> GPLGSPNSEEEASVSVWDEEEDGATFTVTSRQYRPLDPLAPLPPPRSSRRLRAGTLEALVRHLLDARTAGADMMFTPALLATHRAFTSTPALFGLVADRLEALESYPPGELERTTGVAISVLSTWLASHPEDFGSEVKGQLDRLESFLLRTGYAAREGVVGGSADLIRNLRARVDPRAPDLPKPLALPGDSPADPTDVLVFLADHLAEQLTLLDAELFLNLIPSQCLGGLWGHRDRPGHSHLCPSVRATVTQFNKVAGAVVSSVLGATSIGEGPREVTVRPLRPPQRARLLEKWIRVAEECRLLRNFSSVYAVVSALQSSPIHRLRAAWGETTRDSLRVFSSLCQIFSEEDNYSQSRELLTQEVKPQPPVEPHSKK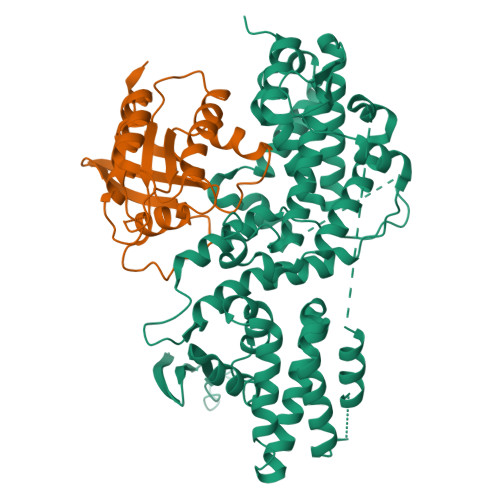APRSGFRGGGVVPYLGTFLKDLVMLDAASKDELENGYINFDKRRKEFAILSELLRLQKECRGYDLRPNSDIQQWLQGLQPLTEAQSHRVSCEVEPPG;> GSMSKKPTAGPALHKVIMVGSGGVGKSALTLQFMYDEFVEDYEPTKADSYRKKVVLDGEEVQIDILDTAGQEDYAAIRDNYFRSGEGFLCVFSITDDESFQATQEFREQILRVKNDESIPFLLVGNKCDLNDKRKVPLSECQLRAQQWAVPYVETSAKTRENVDKVFFDLMREIRSRKTEDSKATSGRAKDRCKKRRLKCTLL pmcAntibiotic resistance mediated by β-lactamase-producing bacteria has become one of the major threats to global health. This phenomenon has substantially reduced the efficacy of β-lactam drugs, which are the most commonly prescribed antibiotics worldwide. β-Lactamases (EC.3.5.2.6) are a group of enzymes that can hydrolyze the amide bond of the β-lactam ring, thus making the antibiotics inactive. One such residue, at position 105 (standard Ambler numbering), is suggested to play an important role in substrate discrimination of class A enzymes. Interestingly, BlaC, the β-lactamase from Mycobacterium tuberculosis, possesses Ile at this position, sparking the question about the evolutionary preference for this amino acid. Mutation of Ile105 to Arg in the β-lactamase BlaC simultaneously enhances activity for carbenicillin and the ability to evade clavulanic acid inhibition.

Comparison between BlaC I105R and wild-type structures indicates a minor repositioning of the active site residues with one important difference. The newly introduced arginine at position 105 adopts a conformation that differs from the isoleucine in the WT, moved away from the active site. Consequently, the access to the active site is broadened. In principle, this would allow for easier accommodation of both substrate and inhibitor molecules, but it can also lead to an augmented dissociation rate of the initial Michaelis complex in case interactions between active residues and substrate or inhibitor have weakened. Furthermore, we investigated whether any structural changes in I105R would be detectable in solution using nuclear magnetic resonance (NMR) spectroscopy. In agreement with the observation from the crystal structure, only the 102 to 106 loop, harboring the mutation site, experienced large chemical shift perturbations. In line with the observed MIC value, BlaC I105R showed improved activity (kcat/KMapp) for carbenicillin (2.7-fold increase) but impaired hydrolysis of nitrocefin and ampicillin (4- and 3-fold reduction, respectively). The positively charged guanidinium group of the arginine side chain might act as a “fishing pole” in attracting negatively charged carbenicillin molecules through the carboxylate group on the C6 atom. However, even long and charged residues, like Arg, can serve as a viable replacement, as demonstrated in BlaC.

>[2x]GDLADRFAELERRYDARLGVYVPATGTTAAIEYRADERFAFCSTFKAPLVAAVLHQNPLTHLDKLITYTSDDIRSRSPVAQQHVQTGMTIGQLCDAAIRYSDGTAANLLLADLGGPGGGTAAFTGYLRSLGDTVSRLDAEEPELNRDPPGDERDTTTPHAIALVLQQLVLGNALPPDKRALLTDWMARNTTGAKRIRAGFPADWKVIDKTGTGDYGRANDIAVVWSPTGVPYVVAVMSDRAGGGYDAEPREALLAEAATCVAGVLA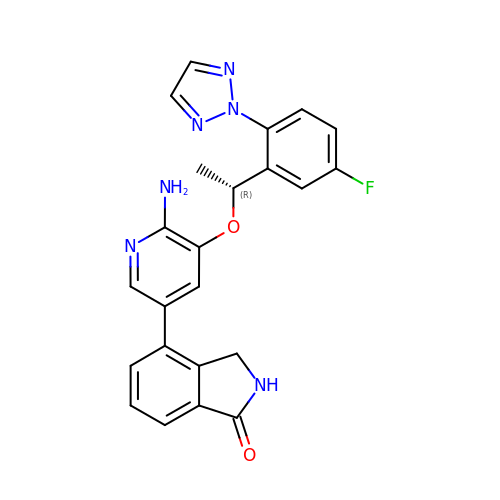4-(6-amino-5-{(1R)-1-[5-fluoro-2-(2H-1,2,3-triazol-2-yl)phenyl]ethoxy}pyridin-3-yl)-2,3-dihydro-1H-isoindol-1-one | C23 H19 F N6 O2 | CKJMFMVVGMXESQ-CYBMUJFWSA-N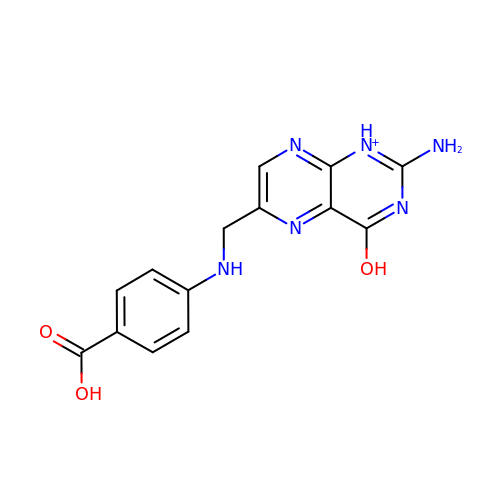2-AMINO-6-[(4-CARBOXY-PHENYLAMINO)-METHYL]-4-HYDROXY-PTERIDIN-1-IUM | C14 H13 N6 O3 | JOAQINSXLLMRCV-UHFFFAOYSA-O>[42x]HEFAELFYRTYIVTPDQAGFQLSIRRNLVWEGWTGEGLSGEKQEISKRNILQGLLDYTTLETNSTELIPVIQSGENDEQFIDPSVLPAQTVKQGKDTFDTNFLKFSENGEGFNLLMLAQTPSRLKKGSMTFTDSLDSRIALKQLLISVTKGGTTELFALDVNRDQYAAYTATREYNFRLMQLKFHTSLGLGEESTTVAGAESALLKDLFDLGYRIELDVKVDGEMNVENGNGDTSLRALRLARVFDKEGKEIALTDSRVSAALSGLTVTGVGYSLEARLTNINQLEMGLLIDSDVQKQGFMIPTLPPLVIVKPAMVEDDKTYPRLEALTTAYRIQQMRNNAVTTLLNRADTLKSYLGVGVPHPIESNLGLEGVGQYYVRPYYNEATIDVLNDLNNLTSAAKQTDIQGLIVSKINEMVYTADQLTGYTAALEAAFSGRSPKPHVAIGTDMRLPQYIQINGDDRTVGIGYDYTIARISDLRMKDKIVMTFILPNESEPHPLQHGVLGFIPEYLVDFNMIRNQRIGREIRLTPRYRYFNFLPIMLVINVINLEEAIAQRTALDVNETQVTPAS

The Klebsiella jumbo myophage ϕKp24 displays an unusually complex arrangement of tail fibers interacting with a host cell. We observe the tail fibers are branched and rearranged dramatically upon cell surface attachment. This complex configuration involves fourteen putative tail fibers with depolymerase activity that provide ϕKp24 with the ability to infect a broad panel of capsular polysaccharide (CPS) types of Klebsiella pneumoniae. In this study, we combine cryo-electron microscopy methods, protein structure prediction methods, molecular simulations, microbiological and machine learning approaches to explore the capsid, tail, and tail fibers of ϕKp24. We determine the structure of the capsid and tail at 4.1 Å and 3.0 Å resolution.

The hexamers and pentamers of ϕKp24 are made up of copies of the same major capsid protein (MCP, gp372, accession number QQV92002). Gp372 contains 597 amino acids and is to our knowledge the largest MCP currently described in any phage. It consists of three major parts: a “triangular body” (gray triangle, dotted box, residues 28–88, 314–597); an “arm” (blue oval, blue, residues 89-166); and a “hand” (orange oval, orange, residues 167–313). Briefly, models of the hexamer and pentamer assemblies were first constructed via rigid docking of the predicted gp372 structure and subsequently refined to our 4.1 Å map using molecular dynamics flexible fitting (MDFF). The triangular body of the MCPs interacts primarily with the triangular bodies of the MCPs directly adjacent and within the same hexamer. These interactions include a series of complimentary salt bridges between residue R477 and E442 on the clockwise neighbor, as well as residue R583 and both D419 and D587 on the clockwise neighbor. The triangular body also interacts strongly with the hand region of its clockwise neighbor through a series of salt bridges, including K380/E220, E398/R190, R554/E313, and R558/D163. In addition to these interactions formed between MCPs within the same hexamer, the hand region also mediates strong interactions with the hand region of an MCP from an adjacent hexamer. These involve a large cluster of charged residues, including E201, K210, K247, D249, E251, D260, and R264, which form complementary interactions. Finally, compared to other known phage capsid structures, the MCP of ϕKp24 displayed a structural feature that has, to our knowledge, not been previously reported: each of the six long C-terminal loops (residues Q582-S597) participate in the formation of a central helical pore with an outer diameter of ~2 nm.>MKTPWKVLLGLLGAAALVTIITVPVVLLNKGTDDATADTRKTYTLTDYLKNTYRLKLYSLRWISDHEYLYKQENNILVFNAEYGNSSVFLENSTFDEFGHSINDYSISPDGQFILLEYNYVKQWRHSYTASYDIYDLNKRQLITEERIPNNTQWVTWSPVGHKLAYVWNNDIYVKIEPNLPSYRITWTGKEDIIYNGITDWVYEEEVFSAYSALWWSPNGTFLAYAQFNDTEVPLIEYSFYSDESLQYPKTVRVPYPKAGAVNPTVKFFVVNTDSLSSVTNATSIQITAPASMLIGDHYLCDVTWATQERISLQWLRRIQNYSVMDICDYDESSGRWNCLVARQHIEMSTTGWVGRFRPSEPHFTLDGNSFYKIISNEEGYRHICYFQIDKKDCTFITKGTWEVIGIEALTSDYLYYISNEYKGMPGGRNLYKIQLSDYTKVTCLSCELNPERCQYYSVSFSKEAKYYQLRCSGPGLPLYTLHSSVNDKGLRVLEDNSALDKMLQNVQMPSKKLDFIILNETKFWYQMILPPHFDKSKKYPLLLDVYAGPCSQKADTVFRLNWATYLASTENIIVASFDGRGSGYQGDKIMHAINRRLGTFEVEDQIEAARQFSKMGFVDNKRIAIWGWSYGGYVTSMVLGSGSGVFKCGIAVAPVSRWEYYDSVYTERYMGL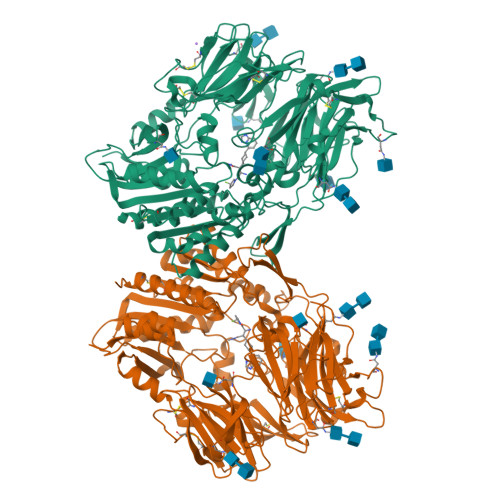PTPEDNLDHYRNSTVMSRAENFKQVEYLLIHGTADDNVHFQQSAQISKALVDVGVDFQAMWYTDEDHGIASSTAHQHIYTHMSHFIKQCFSLP[2x]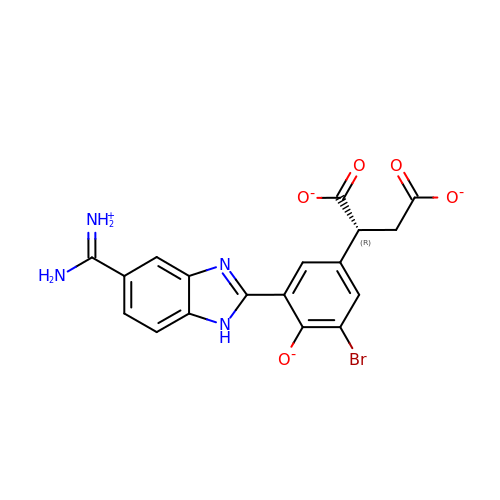2-(3-{5-[AMINO(IMINIO)METHYL]-1H-BENZIMIDAZOL-2-YL}-5-BROMO-4-OXIDOPHENYL)SUCCINATE | C18 H13 Br N4 O5 | SJMNJNRKVVVGRB-SECBINFHSA-L>MAFAISKRNATLFLVTLLLISVPLSSSTLQQDFVKCLVDNSDVSFPITASFFSPDQNATLFKEELESTAQNLRYLTPSNPKPVFIFEPLYETHVQAAVVCAKKLQLHLRLRSGGHDYEGLSFVAEDETPFVIVDLSKLRQVDVDLDSNSAWAHAGATIGEVYYRIQEKSQTHGFPAGLCSSLGIGGHLVGGAYGSMMRKFGLGADNVLDARIVDANGQILDRAAMGEDVFWAIRGGGGGSFGVILAWKIKLVPVPATVTVFTVTKTLEQDGTKVLYKWEQIADKLDDDLFIRVIISPASKTTKPGNRTISMSYQAQFLGDSNRLLQVMQKSFPELGLTKKDCTEMSWIKSVMYIAGFPNSAAPEALLAGKSLFKNHFKAKSDFVKEPIPVEGLEGLWERFLEEDSPLTIWNPYGGMMSRISESEIPFPHRNGTLFKIQWLSTWQDGKVSEERHMKWIREMYSYMEQYVSKNPRQAYVNYRDLDLGTNEGETDAREWGAKYYKGNFERLVKIKGEFDPDNFFRHEQSVPTKIG[2x]

Among them the berberine bridge enzyme (BBE)2-like proteins (pfam 08031) can be set apart due to their unusual bicovalent attachment of the FAD cofactor. Here, we show that the enzymes catalyze the oxidation of aromatic allylic alcohols, such as coumaryl, sinapyl, and coniferyl alcohol, to the corresponding aldehydes and that AtBBE-like 15 adopts the same fold as vanillyl alcohol oxidase for berberine bridge enzyme and other FAD-dependent oxidoreductases. Furthermore, mass spectrometric analysis has shown that AtBBE-like 15 is located in the cell wall and thus might participate in as yet undefined reactions relevant for the formation of the cell wall. Thus, we suggest that AtBBE-like 13 and AtBBE-like 15 participate in the adaptation of the extracellular monolignol pool prior to polymerization and are thus involved in cell wall formation required during certain growth phases and in response to stressors.

Protein crystals were obtained using sitting drop conditions yielding diffraction data to 2.1 Å. AtBBE-like 15 adopts the same fold as other BBE-like enzymes, i.e. the VAO-fold that is characterized by a FAD-binding and a substrate-binding domain (shown in green and orange, respectively). The FAD cofactor is bicovalently linked to the peptide chain via a covalent bond of His-115 to the 8α-methyl group and of Cys-179 to the C6-position of the isoalloxazine ring. In the case of AtBBE-like 15, the gatekeeper residue is a leucine (Leu-182), and thus oxygen reactivity is suppressed because the side chain blocks access to the oxygen pocket. Tyr-117 and Gln-438 are engaged in a hydrogen bond on the si-side of the isoalloxazine ring (2.6 Å). Therefore, these residues were defined as substrate coordination motif. The hydroxyl groups of Tyr-117, Tyr-479, and Tyr-193 point toward the active site with distances to the N5 locus of 4.8, 4.6, and 5.0 Å, respectively. The ϵ-amino group of Lys-436 is located 3.1 Å above the plane of the aromatic ring of Tyr-193 and engages in a cation-π interaction. This arrangement of Tyr-479, Tyr-193, and Lys-436 presumably favors deprotonation of the phenolic hydroxyl group of Tyr-193 and activates this residue as a putative active site base, and thus these residues were defined as a catalytic base motif. The docking result suggests that the orientation of the allylic alcohol toward the proposed catalytic base Tyr-193 is possible, although the aromatic ring is located in the hydrophobic pocket, and thus this orientation is consistent with the productive catalysis found for AtBBE-like 15 with this ligand.>MAGMKTASGDYIDSSWELRVFVGEEDPEAESVTLRVTGESHIGGVLLKIVEQINRKQDWSDHAIWWEQKRQWLLQTHWTLDKYGILADARLFFGPQHRPVILRLPNRRALRLRASFSQPLFQAVAAICRLLSIRHPEELSLLRAPEKKEKKKKEKEPEEELYDLSYHMLSRPQPPPDPLLLQRLPRPSSLSDKTQLHSRWLDSSRCLMQQGIKAGDALWLRFKYYSFFDLDPKTDPVRLTQLYEQARWDLLLEEIDCTEEEMMVFAALQYHINKLSQSGEVGEPAGTDPGLDDLDVALSNLEVKLEGSAPTDVLAEGLNPYGLVAPRFQRKF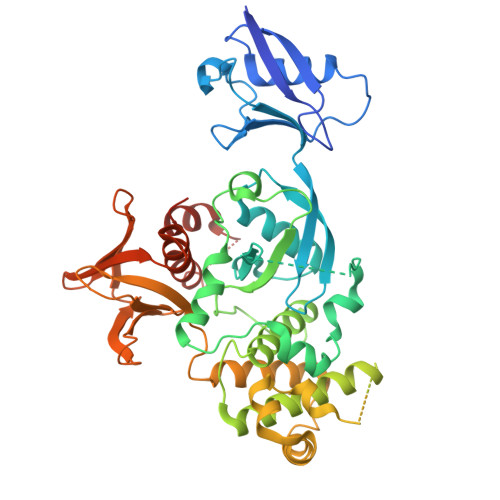KAKQLTPRILEAHQNVAQLSLAEAQLRFIQAWQSLPDFGISYVMVRFKGSRKDEILGIANNRLIRIDLAVGDVVKTWRFSNMRQWNVNWDIRQVAIEFDEHINVAFSCVSASCRIVHEYIGGYIFLSTRERARGEELDEDLFLQLTGGHEAFLEHHHHHH[2x]> GPLGSPLIGEIGPETYSDYMSAGIPLAYIFAETAEERKELSDKLKPIAEAQRGVINFGTIDAKAFGAH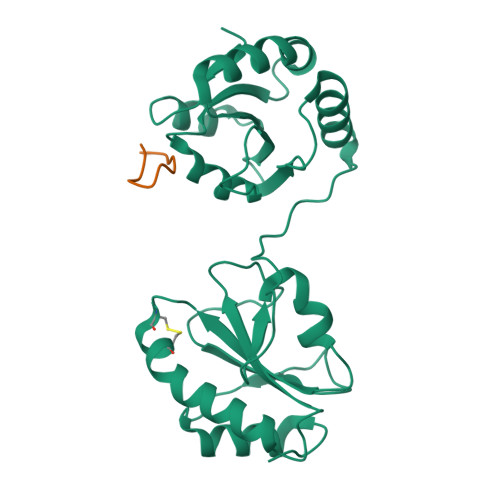AGNLNLKTDKFPAFAIQEVAKNQKFPFDQEKEITFEAIKAFVDDFVAGKIEPSIKSEPIPEKQEGPVTVVVAKNYNEIVLDDTKDVLIEFYAPWCGHCKALAPKYEELGALYAKSEFKDRVVIAKVDATANDVPDEIQGFPTIKLYPAGAKGQPVTYSGSRTVEDLIKFIAENGKYKAA;> GKTKEGVLYVG>[4x]AVTGQVDVKLNISTGCTVGGSQTEGNMNKFGTLNFGKTSGTWNNVLTAEVASAATGGNISVTCDGTDPVDFTVAIDGGERTDRTLKNTASADVVAYNVYRDAARTNLYVVNQPQQFTTVSGQATAVPIFGAIAPNTGTPKAQGDYKDTLLVTVNF

Adhesive pili assembled through the chaperone–usher pathway are hair-like appendages that mediate host tissue colonization and biofilm formation of Gram-negative bacteria. The formation of this biofilm is mediated by Csu pili assembled through the archaic chaperone–usher CsuC–CsuD pathway. The Csu pilus comprises the major subunit CsuA/B that forms the pilus rod, adaptor subunits CsuA and CsuB, and the two-domain tip adhesin CsuE that binds to various substrates using exposed hydrophobic finger-like loops. The rod-forming CsuA/B subunit deviates from the standard Ig-fold and adopts an unusual architecture featuring two prominent hairpins A′–A″ and B–B′ protruding from the β-sheet.

Here, we present the cryo-electron microscopy structure of the prototypical archaic Csu pilus that mediates biofilm formation of Acinetobacter baumannii—a notorious multidrug-resistant nosocomial pathogen. The structure of the Csu pilus rod was determined to an overall resolution of 3.4 Å. The Csu pilus is a thin (around 23 Å) left-handed filament with a helical rise (z) of 28.0 Å and rotation between subunits (φ) of −153°. Pilins are tilted around 60° relative to the helical axis and about 69° relative to each other, resulting in a zigzag appearance of pili when viewed in sideways projection. In contrast to their classical counterparts, the subunits in Csu rods are linked together not by one, but by two binding mechanisms. First, the incoming CsuA/BN+1 pilin subunit inserts its donor strand GdN+1 into the hydrophobic groove of the preceding CsuA/BN subunit. In the pilus, CsuA/BN+1 not only provides GdN+1 to CsuA/BN, but also inserts its A′–A′′ hairpin into a pocket in CsuA/BN between β-strands B and E2 and loop D–D′. Moreover, the GdN+2 of the third subunit CsuA/BN+2 that complements CsuA/BN+1 binds through its protruding N-terminal part to β-strands A′′ and B in CsuA/BN. Finally, residues in β-strand A and loop A–A′ in CsuA/BN+1 form several contacts with residues in the A′′–B loop at the bottom of CsuA/BN, thereby bridging the two main binding sites to form a continuous binding surface of 600 Å2 with 41 interacting residues and 13 hydrogen bonds. Thus, the clinch contact confers pilus rigidity and determines the trajectory of subunit movement during clinch formation or pilus stretching.> SMVAWFAFDPGSAHSDIILSNDNLTVTCSSYDDRVVLGKTGFSKGIHYWELTVDRYDNHPDPAFGVARMDVMKDVMLGKDDKAWAMYVDNNRSWFMHNNSHTNRTEGGITKGATIGVLLDFNRKNLTFFINDEQQGPIAFDNVEGLFFPAVSLNRNVQVTLHTGLPVPDFYSSRASIA

The tripartite motif (TRIM) proteins form one of the largest subfamilies of RING-type E3 ubiquitin ligases, comprising more than 80 members. TRIM family members typically contain a RING domain usually catalyzing ubiquitin transfer; one or two B-box domains mediating protein–protein interactions; and a large coiled-coil domain region, which is involved in self-association or oligomerization with other TRIM E3-ligase proteins (Fiorentini et al., 2020, Ozato et al., 2008). About two-thirds of human TRIM proteins feature a PRYSPRY domain, also known as the B30.2 domain, in their C-terminal region. All characterized family members shared the same overall PRYSPRY twisted β-sandwich fold consisting of a 7-stranded and a 6-stranded antiparallel β-sheet.

There are significant variations in the length, conformation, and amino acid composition of the loops connecting the β-strands. For example, we observed a unique 11-residue deletion between β-strands 2 and 3 in the phylogenetically more closely related family members TRIM9 and TRIM67 (Fig. 1A/B and Fig. 2). Compared with the recently determined structures of TRIM7 PRYSPRY with a peptide substrate or a peptidomimetic ligand (Liang et al., 2022, Munoz Sosa et al., 2024), the putative substrate-binding site in the structure of the two phylogenetically closely related family members TRIM9 and TRIM67 was much shallower. This was largely, but not only, due to a distinct orientation of the β5/β6 loop. In TRIM9, this methionine, Met608, packs against Tyr619 on β-strand 6. The equivalent interacting residues in TRIM67 exemplifying this loop collapse are Met680 and Tyr691. That this was seen in both the TRIM9 and TRIM67 structures suggests it is an intrinsic property of this loop in these two closely related homologs, rather than being induced by crystal packing. In summary, our structural data provide a platform for future drug discovery efforts but, importantly, also hint at significant challenges in developing potent small-molecule binders targeting the canonical binding site, especially in cases of particularly shallow surfaces and those partly or largely occluded by either loop collapse (TRIM9/67) or dimerization (TRIM36).>MGSSHHHHHHSSGLVPRGSHMASSTNTLMYLFADDTHHTATSVDYQSNSAIVKNENSVLNVQFQSKKNSYASIVFSPEKPWDWSEFNDFNLAFELANPGTHSVQIYLDISDIDGANYTRSVNVPVGGYNTYYAKLDGHDLATP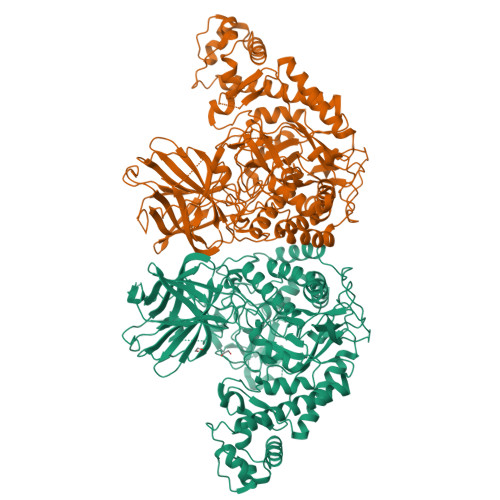DGKENVELNFTSGLRSNPDTWESDEVQFISMWGKKNLNLKGIAKIAISVQSTLHDKELAIKSISLRKNPQFNTAFLTKIVDEFGQNAKQEFAGKVHSEAELLSDKKQEATQLLSKRPTNRSRFGGWAEGPKLEATGYFRTAKYNDKWSLVDPDGYLYLATGIDIIRLANSTTLTGYDFDQALLAKPADAGVTPEDSKGLNQVNKEALKSRFVASQVRKNLFEWLPDYSDTLGKHFGYRKSAHSGPLEHGETYSFYAANLERKYGQNNADYMQKWREVTLDRMITWGFSSLGNWTDPSYYDNQKVPYFANGWIIGDFKTVSSGNDFWGAMPDVFDPEFTVRANETVSVVAKEVKNSPWAVGVFIDNEKSFGRPDSVKSHYGIVINTLGRDAKTVPTKAEFSRLMKEKYTDVAELNKVWHLNLASWAEFDKGVTIDIKNEEQLVDFSILLTAYADKYFSVVNAAMDKYLPNHMYLGARFPDWGMPIEVVKASAKYVDVISFNAYKEGLRDDKWAFLSQFDKPAIIGEFHVGSSDSGLFHPGLIHAANQQDRANMYTDYMNSVIDNPYFIGAHWFQYIDSPITGRAYDGENYNVGFISVTDRPYIEMIEAAKAMNESMYERRFKK[2x]> KPVWAPHPTDGFQVGNIVDIGPDSLTIEPLNQKGKTFLALINQVFPAEEDSKKDVEDNCSLMYLNEATLLHNIKVRYSKDRIYTYVANILIAVNPYFDIPKIYSSETIKSYQGKSLGTMPPHVFAIADKAFRDMKVLKLSQSIIVSGESGAGKTENTKFVLRYLTESYGTGQDIDDRIVEANPLLEAFGNAKTVRNNNSSRFGKFVEIHFNEKSSVVGGFVSHYLLEKSRICVQGKEERNYHIFYRLCAGASEDIRERLHLSSPDNFRYLNRGCTRYFANKETDKQILQNRKSPEYLKAGSLKDPLLDDHGDFIRMCTAMKKIGLDDEEKLDLFRVVAGVLHLGNIDFEEAGSTSGGCNLKNKSTQALEYCAELLGLDQDDLRVSLTTRVMLTTAGGAKGTVIKVPLKVEQANNAR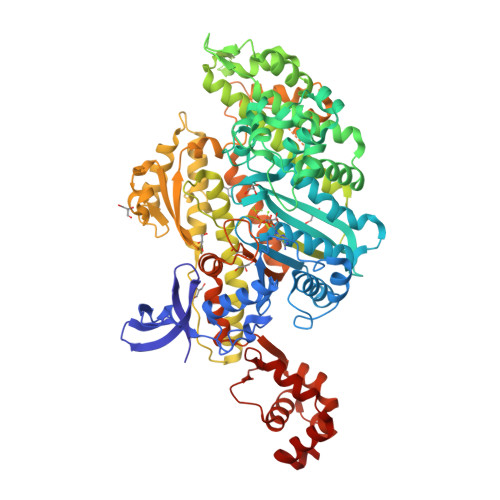DALAKTVYSHLFDHVVNRVNQCFPFETSSYFIGVLDIAGFEYFEHNSFEQFCINYCNEKLQQFFNERILKEEQELYQKEGLGVNEVHYVDNQDCIDLIEARLVGILDILDEENRLPQPSDQHFTSAVHQKHKDHFRLSIPRKSKLAIHRNIRDDEGFIIRHFAGAVCYETTQFVEKNNDALHMSLESLICESRDKFIRELFESSTNNNKDTKQKAGKLSFISVGNKFKTQLNLLLDKLRSTGASFIRCIKPNLKMTSHHFEGAQILSQLQCSGMVSVLDLMQGGFPSRASFHELYNMYKKYMPDKLARLDPRLFCKALFKALGLNEIDYKFGLTKVFFRPGKFAEFDQIMKSDPDHLAELVKRVNHWLI>[2x]GSHMEFDERDRVQKKTFTKWVNKHLIKHWRAEAQRHISDLYEDLRDGHNLISLLEVLSGDSLPREKGRMRFHKLQNVQIALDYL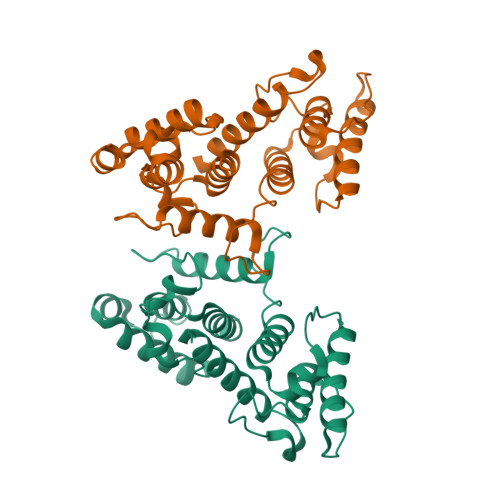RHRQVKLVNIRNDDIADGNPKLTLGLIWTIILHFQISDIQVSGQSEDMTAKEKLLLWSQRMVEGYQGLRCDNFTTSWRDGRLFNAIIHRHKPMLIDMNKVYRQTNLENLDQAFSVAERDLGVTRLLDPEDVDVPQPDEKSIITYVSSLYDAMPRVPGAQEF>[4x]GMDYQEYQQFLARINTARDACVAKDIDVDLLMARHDYFGRELCKSLNIEYRNDVPFIDIILDIRPEVDPLTIDAPHITPDNYLYINNVLYIIDYKVSVSNESSVITYDKYYELTRDISDRLSIPIEIVIIRIDPVSRDLHINSDRFKELYPTIVVDINFNQFFDLKQLLYEKFGDDEEFLLKVA

Bunyaviruses are a large family of segmented RNA viruses which, like influenza virus, use a cap-snatching mechanism for transcription whereby short capped primers derived by endonucleolytic cleavage of host mRNAs are used by the viral RNA-dependent RNA polymerase (L-protein) to transcribe viral mRNAs. Here we structurally and functionally characterize a similar endonuclease in La Crosse orthobunyavirus (LACV) L-protein. We expressed N-terminal fragments of the LACV L-protein and found that residues 1-180 have metal binding and divalent cation dependent nuclease activity analogous to that of influenza virus endonuclease. As expected from the initial sequence analysis, LC183 has exactly the same core, cation-binding fold as found in PA-Nter and more generally in the PD-(D/E)xK nuclease superfamily.

A second structure, at 2.3 Å resolution (R-factor/R-free = 0.177/0.216), was obtained after soaking the crystals with the diketo acid inhibitor 2,4-dioxo-4-phenylbutanoic acid (DPBA). This is a member of the family of 4-substituted 2,4-dioxobutanoic acids which are known inhibitors of influenza virus endonuclease. The two ions are separated by 3.8 Å and have overlapping octahedral co-ordination. The inhibitor DPBA binds tightly to the two metal ions in the active site with three of its oxygen atoms replacing three water molecules in the two metal ion co-ordination. The phenyl group of the inhibitor is less well-defined in the electron density indicative of some residual rotational flexibility. This is indicative of the fact that no direct interactions are made between the DPBA and residues of the protein. In the case of LC183, Asp52, one of the acidic ligands of cation site 2, is on a flexible loop. In the inhibitor bound structure, the loop is in a closed conformation and Asp52 contributes to binding the second manganese. Furthermore metal binding to site 2 requires closure of the Asp52 loop and may be co-operatively dependent on binding of a nucleic acid substrate or metal binding inhibitor such as DPBA.>MNLLSDKNVAIIGGGPVGLTMAKLLQQNGIDVSVYERDNDREARIFGGTLDLHKGSGQEAMKKAGLLQTYYDLALPMGVNIADKKGNILSTKNVKPENRFDNPEINRNDLRAILLNSLENDTVIWDRKLVMLEPGKKKWTLTFENKPSETADLVILANGGMSKVRKFVTDTEVEETGTFNIQADIHQPEINCPGFFQLCNGNRLMASHQGNLLFANPNNNGALHFGISFKTPDEWKNQTQVDFQNRNSVVDFLLKKFSDWDERYKELIHATLSFV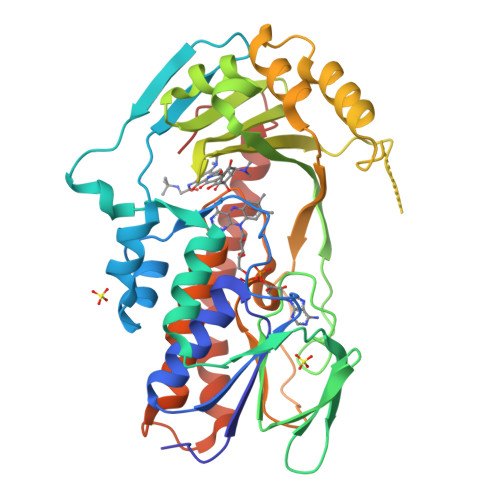GLATRIFPLEKPWKSKRPLPITMIGDAAHLMPPFAGQGVNSGLVDALILSDNLADGKFNSIEEAVKNYEQQMFIYGKEAQEESTQNEIEMFKPDFTFQQLLNV[4x]>MPTDLERRRAIDTAASMYLAEEPLDMSLLAERLGVGRATLYRWVGNR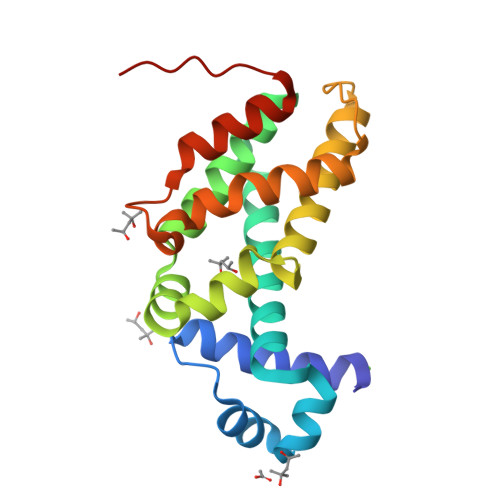DELLGTVLAEATERTYRKAMSQASGQGPEYILDVFGRVMRSVESSTELRALTKREPMVFIKLAMMPGSIESISASITAEILQSQVDAGQLTITLSPQVLGEALVRICDVHLYAPLLGREKAEIETALDLIALLLGVTRNHHHHHH[2x]>[2x]MGWSHPQFEKENLYFQGSATEKYYIRDAITKPAVHHESYQKLWETKWKKPCEMGVYPFMFGSIKDFEPVAQEIIKKGLKEPYDWDEYAQMYFPKAEELAKIAEEAEAAGEKEKASEYYLRSSAVYRISRFPTPRSEKQKYAWRKGCEVFYKGAALMEYPIKEVRIPHKHGIEGEGDVVPVNFLLPPNASETSPVPCVLIITGLDGYRTELAV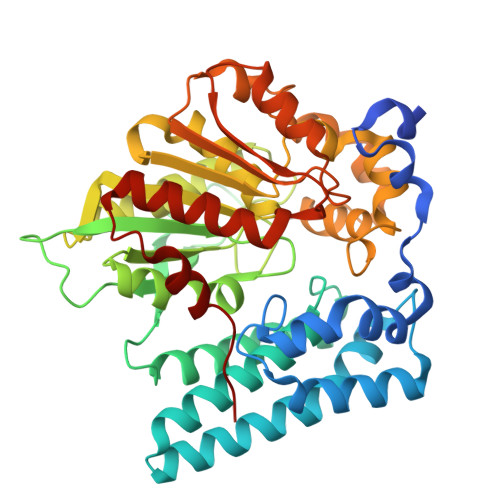WQQGWRSKGVATVIAEIPGTGDSPALRQDPTSPDRQWSSVLDWIESQKAVDSKKIVAWGFSTGGYYALRMAHTHKDRLLATISLGGGAHHMFDREWLEHANKLEYPFDLSNTLAYKFGYPDLESFIEESSKFSLLNDGTLQKPCTKVLLVNGNDDEIFPIDDMFVSLENGQPKLARMVKGKKHMGEPESFSIILEWIHKLLGLDGKIKEQLAMIPSRTK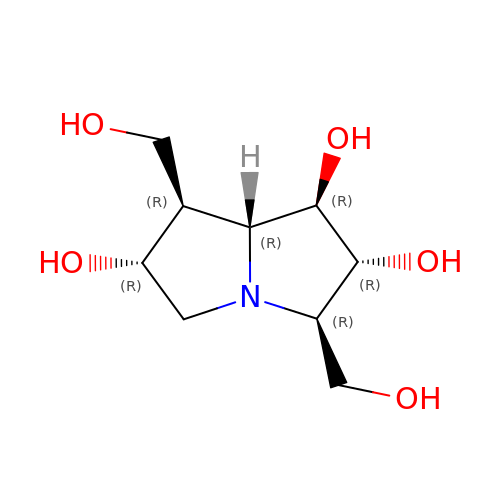(1R,2R,3R,6R,7R,7AR)-3,7-BIS(HYDROXYMETHYL)HEXAHYDRO-1H-PYRROLIZINE-1,2,6-TRIOL | C9 H17 N O5 | WQQQECZSNNTNJJ-FJYMVOSHSA-N>MAKGGSRVSNPAVMAQEEEDVRDYNLTEEQKAIKAKYPPVNRKYEYLDHTADVQLHAWGDTLEEAFEQCAMAMFGYMTDTGTVEPLQTVEVETQGDDLQSLLFHFLDEWLYKFSADEFFIPREVKVLSIDQRNFKLRSIGWGEEFSLSKHPQGTEVKAITYSAMQVYNEENPEVFV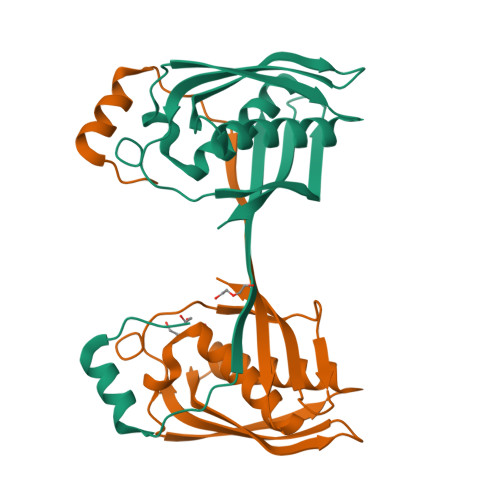IIDILEHHHHHH[2x]>MSDISKASLPKAIFLMGPTASGKTALAIELRKILPVELISVDSALIYKGMDIGTAKPNAEELLAAPHRLLDIRDPSQAYSAADFRRDALAEMADITAAGRIPLLVGGTMLYFKALLEGLSPLPSADPEVRARIEQQAAEQGWESLHRQLQEVDPVAAARIHPNDPQRLSRALEVFFISGKTLTELTQTSGDALPYQVHQFAIAPASRELLHQRIEQRFHQMLASGFEAEVRALFARGDLHTDLPSIRCVGYRQMWSYLEGEISYD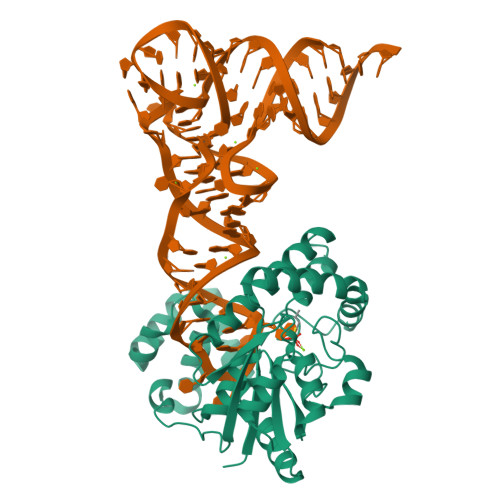EMVYRGVCATRQLAKRQITWLRGWEGVHWLDSEKPEQARDEVLQVVGAIAG[2x]> MAHHHHHHHHENLYFQSRQAFRKFTKSERSKDLIKEAILDNDFMKNLELSQIQEIVDCMYPVEYGKDSCIIKEGDVGSLVYVMEDGKVEVTKEGVKLCTMGPGKVFGELAILYNCTRTATVKTLVNVKLWAIDRQCFQTIMMSTGLIKHTEYMEFLKSVPTFQSLPEEILSKLADVLEETHYENGEYIIRQGARGDTFFIISKGTVNVTREDSP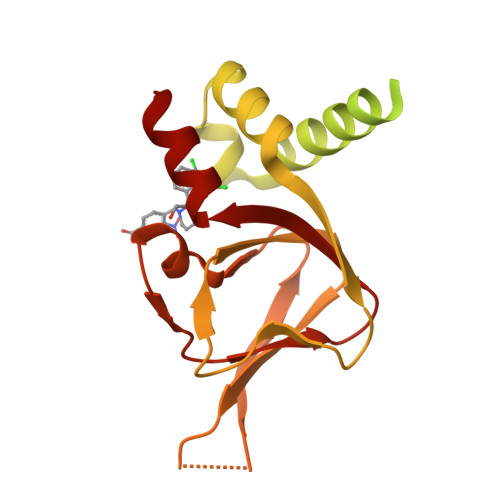SEDPVFLRTLGKGDWFGEKALQGEDVRTANVIAAEAVTCLVIDRDSFKHLIGGL>[2x]MGWKT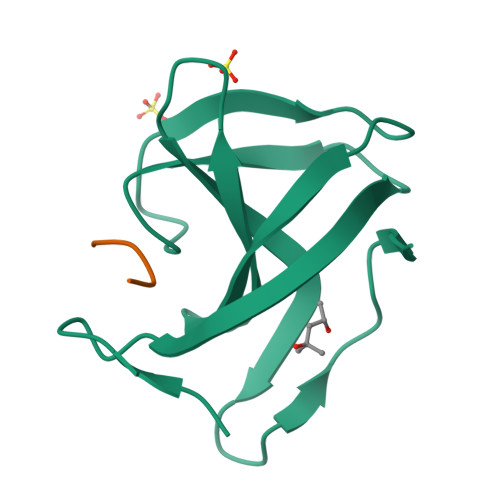NKYGTLYKSESASFTPNTDIITRTTGPFRSMPQSGVLKAGQTIHYDEVMKQDGHVWVGYTGNSGQRIYLPVRTWNKSTNTLGVLWGTIK;>GGGGG[2x]>[2x]GGGRMEHVDSDFAPIRRSKKVVDSDKIVKAISDDLEQKNFTVLRKLNLVPIKKSVSSPKVCKPSPVKERVDHVFYQKFKSMALQELGTNYLSISYVPSLSKFLSKNLRSMKNCIVFFDKVEHIHQYAGIDRAVSETLSLVDINVVIIEMNDYLMKEGIQSSKSKECIESMGQASYSGQLDFEASEKPSNHTSDLMMMVMRKINNDESIDHIVYFKFEQLDKLSTSTIIEPSKLTEFINVLSVLEKSNNIA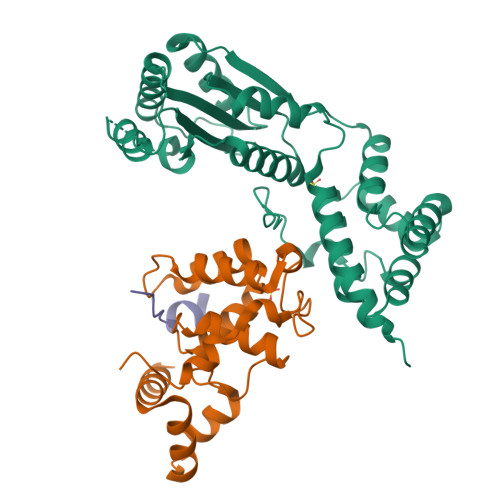FKVLIYSNNVSISSLLSTSLKKKLNTKYTVFEMPILTCAQEQEYLKKMIKFTFDSGSKLLQSYNSLVTCQLNNKESNLAIFFEFLKVFPHPFTYLFNAYTEIIVQSRTFDELLDKIRNRLTIKNYPHSAYNFKKNQRLPLKLTRKVHDR;>GASNSYAIPENELLDEDTMNFISSLKNDLSNISNSLPFEYPHEIAEAIRSDFSNEDIYDNIDPDTISFPPKIATTDLFLPLFFHFGSTRQFMDKLHEVISGDYEPSQAEKLVQDLCDETGIRKNFSTSILTCLSGDLMVFPRYFLNMFKDNVNPPPNVPGIWTHDDDESLKSNDQEQIRKLVKKHGTGRMEMRKRFFEKDLL[2x];>[2x]FTVLRKLNLVPIK>[2x]STAGKVIKCKAAVLWEEKKPFSIEEVEVAPPKAHEVRIKMVATGICRSDDHVVSGTLVTPLPVIAGHEAAGIVESIGEGVTTVRPGDKV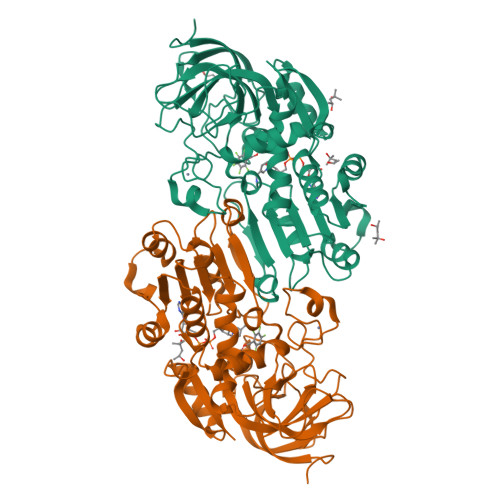IPLFTPQCGKCRVCKHPEGNFCLKNDLSMPRGTMQDGTSRFTCRGKPIHHFLGTSTFSQYTVVDEISVAKIDAASPLEKVCLIGCGFSTGYGSAVKVAKVTQGSTCAVFGLGGVGLSVIMGCKAAGAARIIGIDINKDKFAKAKEVGATECVNPQDYKKPIQEVLTEMSNGGVDFSFEVIGRLDTMVTALSCCQEAYGVSVIVGVPPDSQNLSMNPMLLLSGRTWKGAIFGGFKSKDSVPKLVADFMAKKFALDPLITHVLPFEKINEGFDLLRSGESIRTILTF>[2x]MHHHHHHMANRKLEKMASIDVHLRQLVPGKVSEDDKLVEYDALLLDRFLDILQDLHGEDLRETVQELYEHSAEYEGKHEPKKLEELGSVLTSLDPGDSIVIAKAFSHMLNLANLAEEVQIAYRRRIKKLKKGDFVDESSATTESDLEETFKKLVGDLNKSPEEIFDALKNQTVDLVLTAHPTQSVRRSLLQKHGRIRDCLAQLYAKDITPDDKQELDEALQREI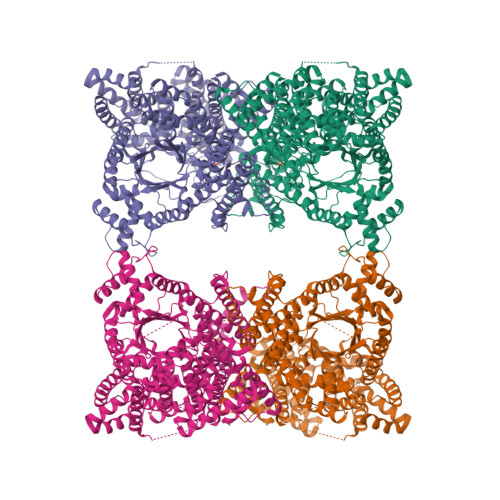QAAFRTDEIKRTPPTPQDEMRAGMSYFHETIWKGVPKFLRRVDTALKNIGIEERVPYNAPLIQFSSWMGGDRDGNPRVTPEVTRDVCLLARMMAATMYFNQIEDLMFEMSMWRCNDELRARADEVHANSRKDAAKHYIEFWKSIPTTEPYRVILGDVRDKLYHTRERAHQLLSNGHSDVPVEATFINLEQFLEPLELCYRSLCSCGDRPIADGSLLDFLRQVSTFGLSLVRLDIRQESDRHTDVLDAITTHLDIGSYREWSEERRQEWLLSELSGKRPLFGSDLPKTEEIADVLDTFHVIAELPADSFGAYIISMATAPSDVLAVELLQRECRVKQPLRVVPLFEKLADLEAAPAAVARLFSVDWYKNRINGKQEVMIGYSDSGKDAGRLSAAWQLYKAQEELVKVAKEYGVKLTMFHGRGGTVGRGGGPTHLAILSQPPDTINGSLRVTVQGEVIEQSFGEEHLCFRTLQRFTAATLEHGMRPPISPKPEWRALLDEMAVVATEEYRSVVFQEPRFVEYFRLATPELEYGRMNIGSRPSKRKPSGGIESLRAIPWIFAWIQTRFHLPVWLGFGSAIRHVIEKDVRNLHMLQDMYQHWPFFRVTIDLIEMVFAKGDPGIAALYDKLLVSEELWPFGEKLRANFEETKKLILQTAGHKDLLEGDPYLKQRLRLRDSYITTLNVCQAYTLKRIRDPSYHVTLRPHISKEIAESSKPAKELIELNPTSEYAPGLEDTLILTMKGIAAGLQNTG>SMFEIKKICCIGAGYVGGPTCSVIAHMCPEIRVTVVDVNESRINAWNSPTLPIYEPGLKEVVESCRGKNLFFSTNIDDAIKEADLVFISVNTPTKTYGMGKGRAADLKYIEACARRIVQNSNGYKIVTEKSTVPVRAAESIRRIFDANTKPNLNLQVLSNPEFLAEGTAIKDLKNPDRVLIGGDETPEGQRAVQALCAVYEHWVPREKILTTNTWSSELSKLAANAFLAQRISSINSISALCEATGADVEEVATAIGMDQRIGNKFLKASVGFGGSCFQKDVLNLVYLCEALNLPEVARYWQQVIDMNDYQRRRFASRIIDSLFNTVTDKKIAILGFAFKKDTGDTRESSSIYISKYLMDEGAHLHIYDPKVPREQIVVDLSHPGVSEDDQVSRLVTISKDPYEACDGAHAVVICTE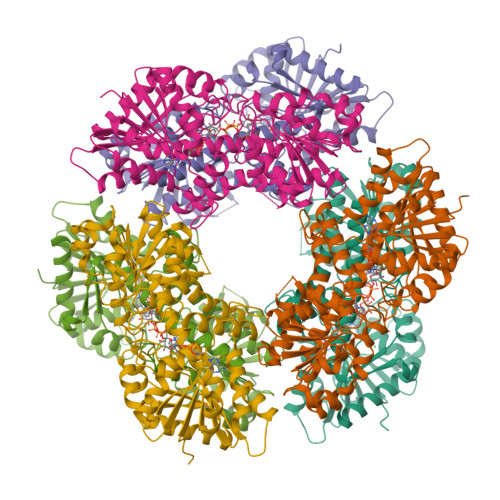WDMFKELDYERIHKKMLKPAFIFDGRRVLDGLHNELQTIGFQIETIGKKV[12x]In the order Corynebacteriales, which includes the important pathogens Mycobacterium tuberculosis and Corynebacterium diphtheriae, the most important murein hydrolase for cell separation is the endopeptidase RipA. We present here the crystal structure of a full-length RipA homologue from Corynebacterium glutamicum, Cg1735, which reveals an unusual mode of autoinhibition. We describe how this autoinhibition is relieved by the conserved transmembrane protein Cg1604 and propose an FtsEX-independent model for septal control of PG hydrolysis via the Cg1604–Cg1735 complex. In this model, two septal TM proteins, Cg1603, with a cytoplasmic N-terminal globular core, and Cg1604, with a C-terminal globular core exposed to the cell envelope, form a signaling complex that couples intracellular cell division events with PG hydrolysis during the last stages of cell separation.

We thus produced the soluble periplasmic domain of Cg1604 (Cg1603 has no extra-cytoplasmic globular domain) and assessed its effect on a PG activity assay of full-length Cg1735. A clear activation effect is observed upon addition of the Cg1604 periplasmic domain to the reaction mixture. To elucidate the activation mechanism, we solved the crystal structure of the periplasmic domain of Cg1604 (residues 36 to 295) by SAD techniques at 2 Å resolution. The structure revealed an extended N-terminal α-helix that connects the N-terminal TM region of the protein (absent in the construct) to a globular domain consisting of a parallel five-stranded β-sheet surrounded by α-helices on both sides. This domain displays the (β/α)5 topology characteristic of receiver domains from bacterial response regulators, except for the insertion of a helical subdomain between β-strands 2 and 3. The globular core of Cg1604 has no obvious groove or pocket that might suggest a putative functional site. However, a patch of surface residues within the subdomain insertion (in the membrane distal face of the protein) is highly conserved in Cg1604 homologs, suggesting that this region might represent a functionally conserved binding site. Indeed, calculations with AlphaFold on the two full-length proteins, Cg1735 and Cg1604, predicted with a relatively high confidence that the Cg1604 subdomain interacts with the CC1 domain of RipA, to form a complex in which the protein–protein interface is highly conserved in both proteins. The crystal structure of monomeric Cg1604 does indeed rule out a putative channel-forming property of the protein. The best crystals of selenomethionine-derived Cg1604 (35 mg/mL) were obtained after 22 d in 30% (w/v) PEG 4 K, 0.2 M MgCl2, 0.1 M TRIS pH 8.5.

> MAKRRGRGAATFAALGFGAAAGIAFGTYVLAPNLPENIDPNAPTSAELVEAETLAEVNAVQADQADSIIDHIVEDVVAGTLTDRPVLVMRTADAEESDVADVSWLLQQAGAINAGSITLEENFFSQDGADQLKSIVANTLPAGAQLSETQLDPGTHAGEALGAALLLNPETGEPLASTAERGLLLNVLRDNGYISYEDGTILPGQVIVMITGDSDGSGDGAFAAETQSLFARALDAQGSGVVVAGRIHTAADTGVIGRLRANPDAAENVSTIDSVNRTWGKMATVLSVREELAGRSGAFGSAASADAASPSLDGTAAAPAQ>SLLTEVETYVLSIIPSGPLKAEIAQRLESVFAGKNTDLEALMEWLKTRPI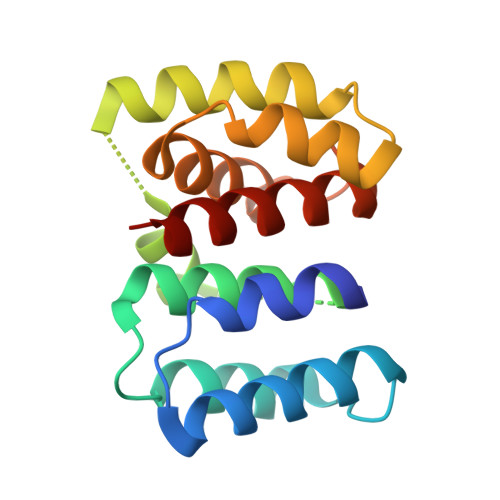LSPLTKGILGFVFTLTVPSERGLQRRRFVQNALNGNGDPNNMDRAVKLYKKLKREITFHGAKEVSLSYSTGALASCMGLIYNRMGTVTTEAAFGLVCATCEQIADSQ[4x]> MASGQDKTHIDYAYELDITVKPDSRVPVFNREFATFTGAGVPLFSLGGGPIRYALAEVLAKFHARRGYYVVETPIIASTELFKVSGHIEFYRNNMYLFDIEGHEFAVKPMNCPYHILLF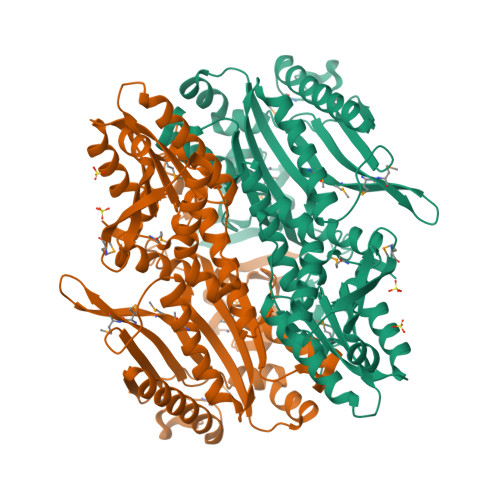LNEVAKHRSKLPLPFKVFEFGRVHRYEPSGSIYGLLRVRGFTQDDAHIIVPGGRVIDVVYDVFEEMKLVLERLFKLGVSSETFKVRLSMSDKSLIGKEFMGSKEEWEGAEEALREAASRINEKYGIDIVELEGEAAFYGPKLDFIMMVEESGVSKEWQMGTIQFDFNLPRRFRLYDVVREEFGIEEVYIIHRALLGSIERFLGVYLEHRRGRMPFTLAPIQFAVIAVKTGGEVDREIEDLASSIAKGLLDKGFRVAVKGSSKTGLSSDVRHIESTAKPAVNVFIGAKEVREKVLDVRVFDLESMKRRRLAIAYGDAADAVENLAAVAEELESPVRSLSGQAPRIPADFSFML> MDTYSVFTTKWKQLTGVDLTLYKEAQMKRRLTSLYEKKGFQSFKDFAAALEKDQALLNETLDRMTINVSEFYRNYKRWEVLETAILPLIKTSRPLKIWSAACSTGEEPYTLAMLLDQQKGLPGYQILATDIDEKALEKAKKGVYQERSLQEVPLSVKDRYFT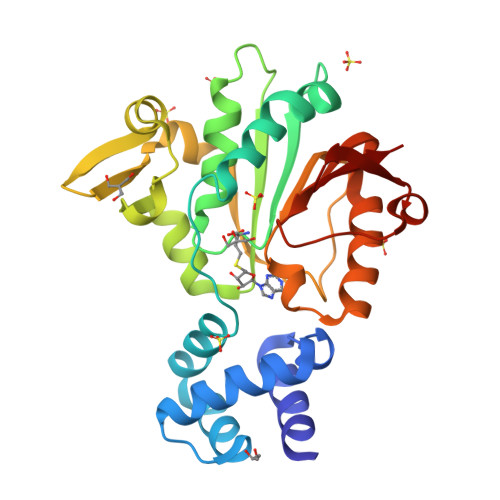QNANRSYEVKTEIKKNITFKKHNLLADRYEQDFDLIVCRNVFIYFTESAKEELYLKMAHSLKKNGVLFVGSTEQIFNPEKFGLVPADTFFYQKR>MKFSKEQFDYSLYLVTDSGMIPEGKTLYGQVEAGLQNGVTLVQIREKDADTKFFIEEALQIKELCHAHNVPLIINDRIDVAMAIGADGIHVGQDDMPIPMIRKLVGPDMVIGWSVGFPEEVDELSKMGPDMVDYIGVGTLFPTLTKKNPKKAPMGTAGAIRVLDALERNNAHWCRTVGIGGLHPDNIERVLYQCVSSNGKRSLDGICVVSDIIASLDAAKSTKILRGLIDKTDYKFVNIGLSTKNSLTTTDEIQSIISNTLKARPLVQHITNKVHQNFGANVTLALGSSPIMSEIQSEVNDLAAIPHATLLLNTGSVAPPEMLKAAIRAYNDVKRPIVFD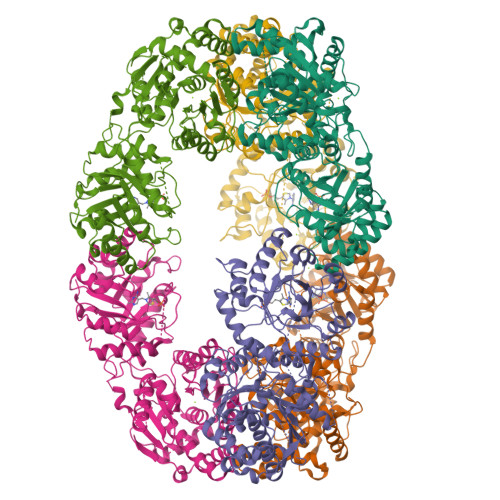PVGYSATETRLLLNNKLLTFGQFSCIKGNSSEILGLAELNKERMKGVDASSGISNELLIQATKIVAFKYKTVAVCTGEFDFIADGTIEGKYSLSKGTNGTSVEDIPCVAVEAGPIEIMGDITASGCSLGSTIACMIGGQPSEGNLFHAVVAGVMLYKAAGKIASEKCNGSGSFQVELIDALYRLTRENTPVTWAPKLTHT[6x]2',3'-DIDEOXYADENOSINE-5'-MONOPHOSPHATE 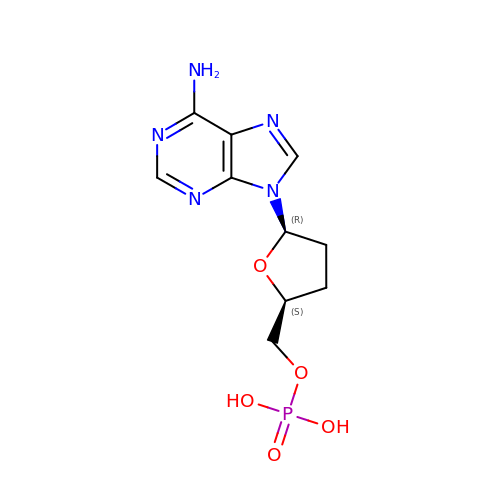| C10 H14 N5 O5 P | PUSXDQXVJDGIBK-NKWVEPMBSA-N> SSQIRQNY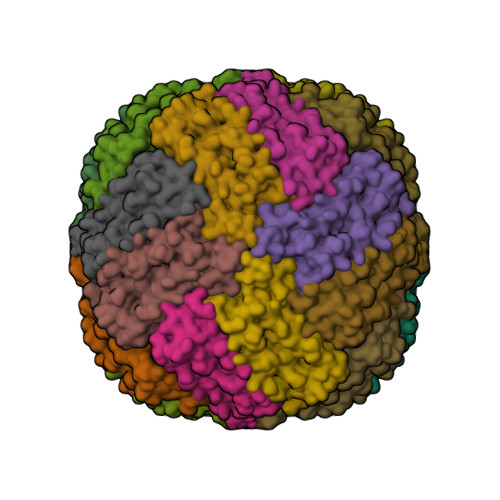STEVEAAVNRLVNLYLRASYTYLSLGFYFDRDDVALEGVCAFFRELAEEKREGAERLLKMQNQRGGRALFQDLQKPSQDEWGTTPDAMKAAIVLEKSLNQALLDLHALGSAQADPHLCDFLESHFLDEEVKLIKKMGDHLTNIQRLVGSQAGLGEYLFERLTLKHD> MATNFFIQPITEEAEAYYPPSVITNKRKDLGVDVYCCSDLVLQPGLNIVRLHIKVACEHMGKKCGFKIMARSSMCTHERLLILANGIGLIDPGYVGELMLKIINLGDTPVQIWAKE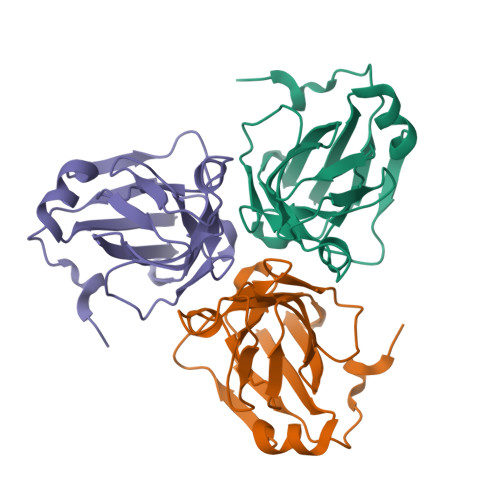CLVQLVAQGDHVPDHINILKRNQIFPLFAPTPRGEGRFGSTGEAGIMRT> ATIKDVAKRANVSTTTVSHVINKTRFVAEETRNAVWAAIKELHYSPSAVARSMKVNHTKSIGLLATSSEAAYFAEIIEAVEKNCFQKGYTLILGNAWNNLEKQRAYLSMMAQKRVDGLLVMCSEYPEPLLAMLEEYRHIPMVVMDWGEAKADFTDAVIDNAFEGGYMAGRYLIERGHREIGVIPGPLERNTGAGRLAGFMKAMEEAMIKVPESWIVQGDFEPESGYRAMQQILSQPHRPTAVFCGGDIMAMGALCAADEMGLRVPQDVSLIGYDNVRNARYFTPALTTIHQPKDSLGETAFNMLLDRIVN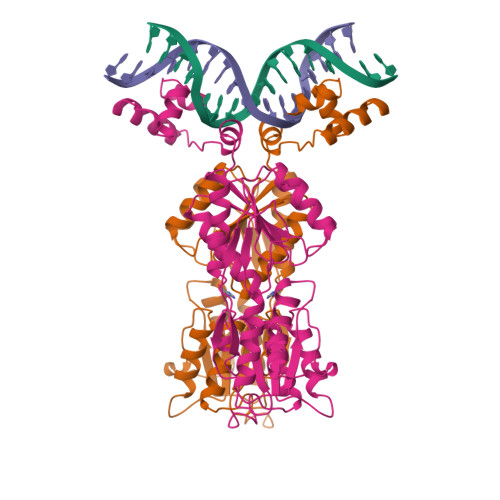KREEPQSIEVHPRLIERRSVADGPFRDYRR>GAMVKSENLSTGNALIDNELDIRGLFRLLWRGKVWPIAIGLLFAVVALGYSYLVKQEWGATSITDKPTVNMLGGYYSQQQFLRNLDARSFSSPQPEQPSISAGAYDEFIMQLAAYDTRRDFWLQTDYYKQRLEGDEKADAALLDELVNNIQFTARDDGKKTNDSVKLVAETSSDSNTLLRQYVVFASQRAANHLNEEIKGAWAARTIFMKSQIKRQEAVAKAIYDREVRSVELALKIAQQQGISRSQTDTPADEIPASEMFLLGRPMLQARLETLQTSGPHYELDYDQNRAMLATLNVGPTLEASFQTYRYLRTPEEPVKRDSPRR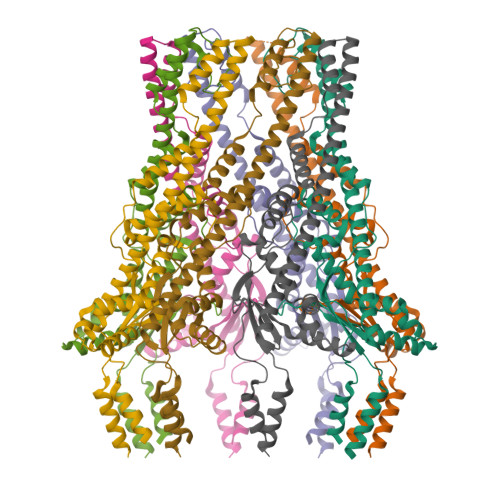AFLMVMWGAIGVLVGAGVALARRLR[8x]>VTAFLGERVTLTSYWRRVSLGPEIEVSWFKLGPGEEQVLIGRMHHDVIFIEWPFRGFFDIHRSANTFFLVVTAANISHDGNYLCRMKLGETEVTKQEHLSVVKPLTLSVHSERSQFPDFSVLTVTCTVNAFPHPHVQWLMPEGVEPAPTAANGGVM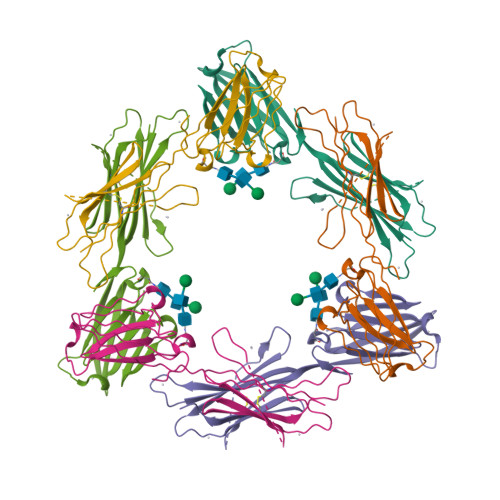KEKDGSLSVAVDLSLPKPWHLPVTCVGKNDKEEAHGVYVSGYLSQ[4x]> PAQPADFQAEVESDTRIQLSWLLPPQERIIMYELVYWAAEDEDQQHKVTFDPTSSYTLEDLKPDTLYRFQLAARSDMGVGVFTPTIEARTAQSTPSAPPQKVMCVSMGSTTVRVSWVPPPADSRNGVITQYSVAYEAVDGEDRGRHVVDGISREHSSWDLVGLEKWTEYRVWVRAHTDVGPGPESSPVLVR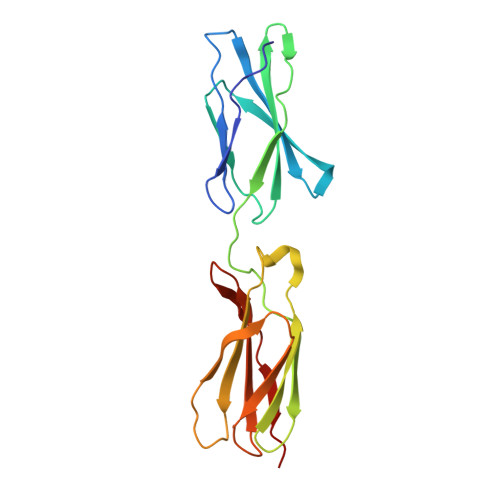TDED7-[[6-[[1-(1-IMINOETHYL)PIPERIDIN-4-YL]OXY]-2-METHYL-BENZIMIDAZOL-1-YL]METHYL]NAPHTHALENE-2-CARBOXIMIDAMID | C27 H31 N6 O | 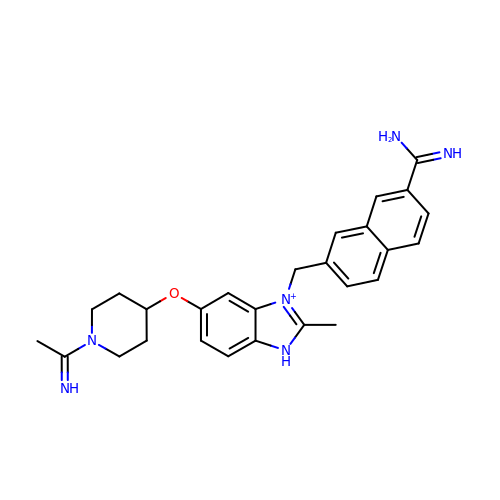JABMRQOJSAZJAD-QRQIAZFYSA-O(8-oxa-2-azaspiro[4.5]decan-2-yl)(2-{[(1S)-1-(pyrazin-2-yl)ethyl]amino}pyrimidin-5-yl)methanone | C19 H24 N6 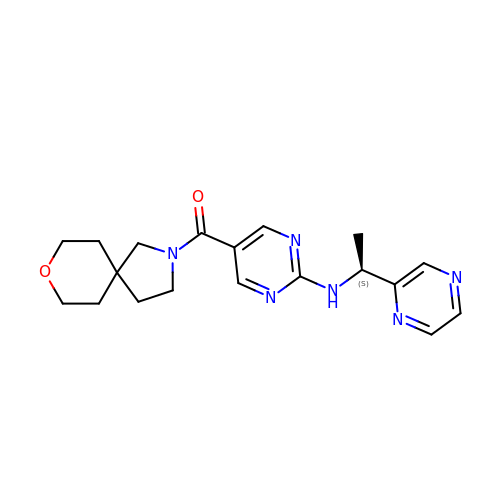O2 | RZEQDKIIEMKNMN-AWEZNQCLSA-N>MVRKGEKKLAKPATTKAANPQPRRRANNRRRSNRTDAPVSKASTVTGFGRGTNDVHLSGMSRISQAVLPAGTGTDGYVVVDATIVPDLLPRLGHAARIFQRYAVETLEFEIQPMCPANTGGGYVAGFLPDPTDNDHTFDALQATRGAVVAKWWESRTVRPQYTRTLLWTSSGKEQRLTSPGRLILLCVGNNTDVVNVSVLCRWSVRLSVPSLENPEETTAPIMTQGSLYNDSLSTNDFKSILLGSTPLDIAPDGAVFQLDRPLSIDYSLGTGDVDRAVYWHLKKFAGNAGTPAGWFRWGIWDNFNKTFTDGVAYYSDEQPRQILLPVGTVCTRVDSEN[90x]

Here we report protein crystal structures of a piscine betanodavirus, the Grouper nervous necrosis virus (GNNV), in four different forms. The overall topological structure of the GNNV CP consists of the N-terminal arm (N-arm) (residues 34−51), the shell domain (S-domain) (residues 52−213), the linker region (residues 214−220) and the protrusion domain (P-domain) (residues 221−338). The S-domain comprises an eight-stranded anti-parallel β-sandwich with three short α-helices, which is a canonical structural feature similar to other virus CPs. The P-domain folds into an independent structure, including eight anti-parallel β-strands and a short α-helix connected with loops of various lengths.

We determine the crystal structure of the T = 3 GNNV-LP using the ab initio method with non-crystallographic symmetry (NCS) averaging and refine the structure to 3.6 Å. The electron density of the icosahedral asymmetric unit (iASU) of the T = 3 GNNV-LP allows modeling of residues 52−338 for subunits A and B, and residues 34−338 for subunit C. The rest of the N-terminal segment of each subunit, which contains N-ARM, the positively charged arginine-rich motif 23RRRANNRRRSN33, is disordered. The ordered N-arm exists along the icosahedral two-fold (I2) interface of the inner surface, and extends its N-terminus to the icosahedral three-fold (I3) axis to form a β-annulus. Residues 36−41 from subunits C1, C10 and C12 are engaged through hydrogen bonding to form a β-annulus structure around the I3 axis. Sixty trimeric S-domains participate in inter-subunit contacts, forming a continuous thin shell of the capsid with an empty inner cavity. Three neighboring P-domains per iASU embrace one another at the quasi three-fold (Q3) axes to form 60 protrusions on the particle surface. There are three S-domains per iASU, and they all share the same calcium-binding structures to facilitate subunit-subunit interactions, similar to those seen in the CP of some RNA plant viruses, such as tombusvirus (DxDxxD) and SeMV (DxxD). The flat conformation of the subunit-C/C dimer is stabilized by two ordered N-arms alone, in contrast to alphanodavirus, where incorporation of the encapsidated RNA participates in the T = 3 quaternary organization. Although the structure of the P-domain can be readily assigned, the protrusions of the GNNV-LP show too poor electron density after NCS-averaging to allow a complete characterization of the morphology of the P-domain, which might be caused by the high flexibility. In addition, a structural comparison reveals that the truncated P-domain contains the rigid P-domain with the disordered linker region, and this linker region of T = 3 GNNV-LP also exhibits large B-factor values. This analysis may provide insights into why the flexible linker region allows the entire solid P-domain to be malleable, resulting in the broken electron density of the P-domain with large B-factor values for the T = 3 GNNV-LP.>MKVWNARNDHLTINQWATRIDEILEAPDGGEVIYNVDENDPREYDAIFIGGGAAGRFGSAYLRAMGGRQLIVDRWPFLGGSCPHNACVPHHLFSDCAAELMLARTFSGQYWFPDMTEKVVGIKEVVDLFRAGRNGPHGIMNFQSKEQLNLEYILNCPAKVIDNHTVEAAGKVFK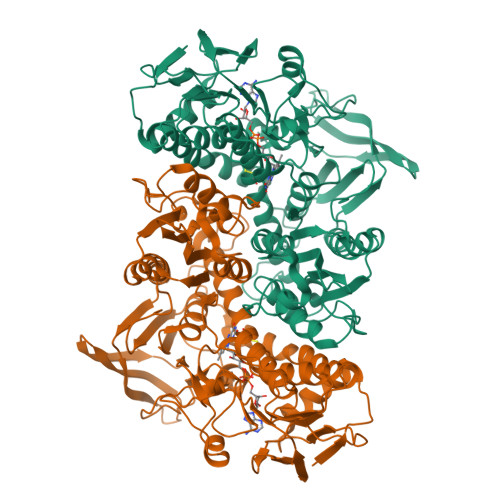AKNLILAVGAGPGTLDVPGVNAKGVFDHATLVEELDYEPGSTVVVVGGSKTAVEYGCFFNATGRRTVMLVRTEPLKLIKDNETRAYVLDRMKEQGMEIISGSNVTRIEEDANGRVQAVVAMTPNGEMRIETDFVFLGLGEQPRSAELAKILGLDLGPKGEVLVNEYLQTSVPNVYAVGDLIGGPMEMFKARKSGCYAARNVMGEKISYTPKNYPDFLHTHYEVSFLGMGEEEARAAGHEIVTIKMPPDTENGLNVALPASDRTMLYAFGKGTAHMSGFQKIVIDAKTRKVLGAHHVGYGAKDAFQYLNVLIKQGLTVDELGDMDELFLNPTHFIQLSRLRAGSKNLVSL[4x]> GHRP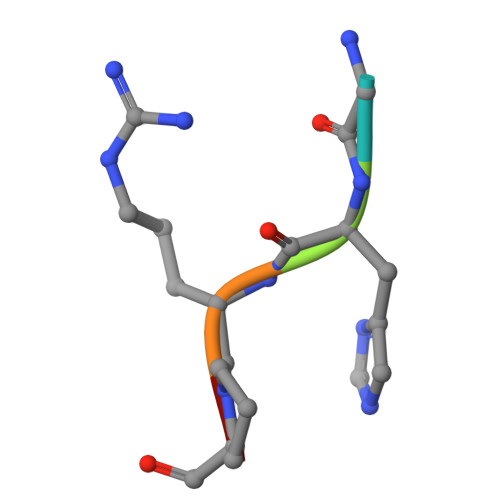X Bacteriophage Casadabanvirus JBD30, from the order Caudoviricetes, is a temperate phage that infects the bacterium Pseudomonas aeruginosa. The virion of bacteriophage JBD30 is composed of an icosahedral capsid, long flexible non-contractile tail, and a baseplate. Using its baseplate, JBD30 attaches to Pseudomonas aeruginosa via the bacterial type IV pilus, whose subsequent retraction brings the phage to the bacterial cell surface.

The tail of bacteriophage JBD30 is a right-handed six-entry helix composed of 45 discs, each built from six major tail proteins (gp44). The twist and rise in between two adjacent discs are 23.5° and 43.2 Å, respectively. The major tail protein of JBD30 consists of a central β-sandwich (residues 8–41, 62–73, 184–256), peripheral α-helix (residues 77–83), decoration domain (residues 88–175), and a long hinge loop (residues 42–62). The inner tail tube diameter, 40 Å, is defined by the β-barrel formed by 24 β-strands, to which each major tail protein contributes four β-strands. The interior of the tube is smooth and round in cross-section. The surface is negatively charged to enable the swift passage of the DNA. As in the tails of phages T5 and λ, the decoration domains of JBD30 major tail protein have an immunoglobulin-like fold, and protrude tangentially from the major tail protein disc. The disc-to-disc contacts are mediated by the hinge loops, each of which is inserted between loops formed by residues 217–227 of two major tail proteins from an adjacent hexamer. We assume that the flexibility of the hinge loop and its interaction with the loops of adjacent major tail proteins enables the bending of the tail, similar to those of phages SPP1 and λ. The JBD30 tail contains a long density inside the tail tube, which was absent in the tail tube reconstructed from empty particles.

> MAQETYFYGQGEIDAAPIVNGVLGKWRWIQDVSAMSIQLAVEKVEHKESYSGQKALVRSFPIGKTATVNITLHSIGPDNLALTLYGKVVAKAAGSVTGEVLPADLVAGDVIRLANFGVSELVITDSASSPAPLDPQYYALRADGAYGEVQLLGLPTPAPTQPFKAAYEYAATKQVGMFTAPQPTVALRYKGINLAEGGAPVIVELYKVATDPLQELALISDGNTVAGMQISGGILLDTSKPDTGDLGRFGRIIQLG>[4x]KGPNLTEISKKITDSNAVLLAVKEVEALLSSIDELAKAIGKKIKNDGSLGDEANHNESLLAGAYTISTLITQKLSKLNG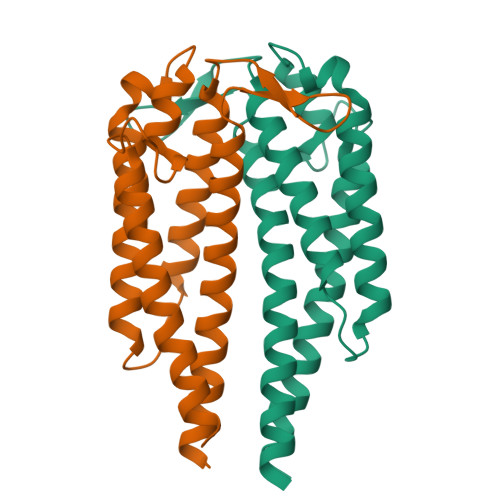SEGLKEKIAAAKKCSEEFSTKLKDNHAQLGIQGVTDENAKKAILKANAAGKDKGVEELEKLSGSLESLSKAAKEMLANSVKELTSPVVAESPKKP> MTLDLPRRFPWPTLLSVCIHGAVVAGLLYTSVHQVIELPAPAQPISVTMVTPADLEPPQAVQPPPEPVVEPEPEPEPIPEPPKEAPVVIEKPKPK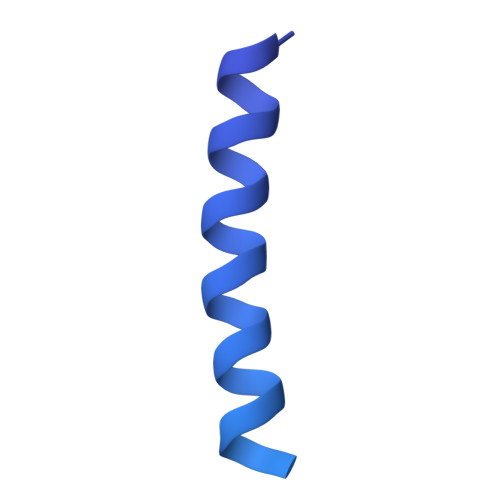PKPKPKPVKKVQEQPKRDVKPVESRPASPFENTAPARLTSSTATAATSKPVTSVASGPRALSRNQPQYPARAQALRIEGQVKVKFDVTPDGRVDNVQILSAKPANMFEREVKNAMRRWRYEPGKPGSGIVVNILFKINGTTEIQGGGSENLYFQGGSAWSHPQFEK>HHHHHHENLYF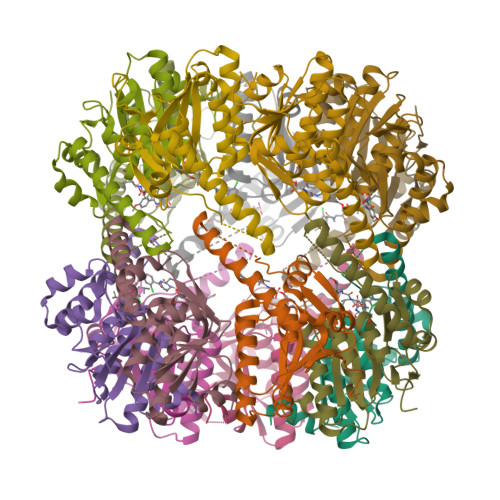QSNMSFDNYLVPTVIEQSGRGERAFDIYSRLLKERIVFLVGPVTDESANLVVAQLLFLESENPDKDIFFYINSPGGSVTAGMSIYDTMNFIKPDVSTLCLGQAASMGAFLLSAGEKGKRFALPNSRIMIHQPLISGGLGGQASDIEIHARELLKIKEKLNRLMAKHCDRDLADLERDTDRDNFMSAEEAKEYGLIDQILENRASLRL[14x]>ADPDPMKNTCKLLVVADHRFYRYMGRGEESTTTNYLIELIDRVDDIYRNTAWDNAGFKGYGIQIEQIRILKSPQEVKPGEKHYNMAKSYPNEEKDAWDVKMLLEQFSFDIAEEASKVCLAHLFTYQDFDMGTLGLAYGGSPRANSHGGVCPKAYYSPVGKKNIYLNSGLTSTKNYGKTILTKEADLVTTHELGHNFGAEHDPDGLAECAPN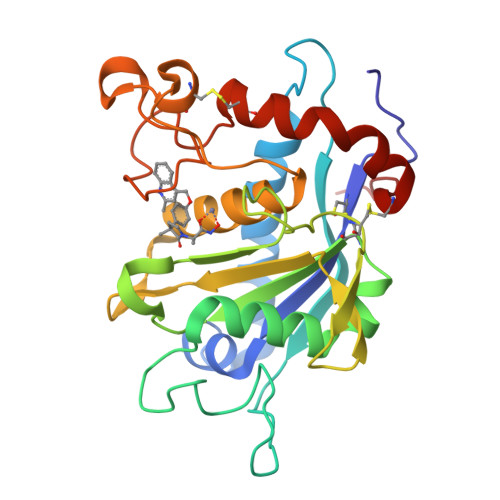EDQGGKYVMYPIAVSGDHENNKMFSQCSKQSIYKTIESKAQECFQERSNA[2x]>[2x]MDARIVNALIGSVYETIRDVLGIEPKTGKPSTVSHIEIPHSLVTVIGITGGIEGSLIYSFSSETALKVVSAMM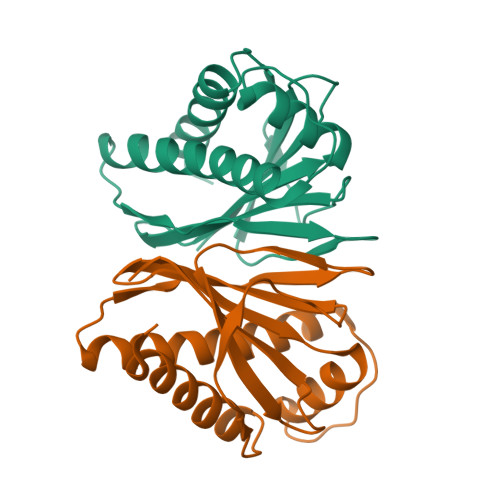GGMEYNQLDELALSAIGELGNMTAGKLAMKLEHLGKHVDITPPTVVSGRDLKIKSFGVILKLPISVFSEEDFDLHLSVKSGG>VHHPPSYVAHLASDFGVRVFQQVA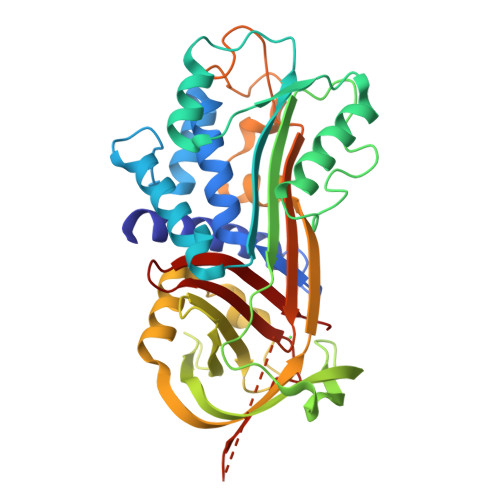QASKDRNVVFSPYGVASVLAMLQLTTGGETQQQIQAAMGFKIDDKGMAPALRHLYKELMGPWNKDEISTTDAIFVQRDLKLVQGFMPHFFRLFRSTVKQVDFSEVERARFIINDWVKTHTKGMISNLLGKGAVDQLTRLVLVNALYFNGQFKTPFPDSSTHRRLFHKSDGSTVSVPMMAQTNKFNYTEFTTPDGHYYDILELPYHGDTLSMFIAAPYEKEVPLSALTNILSAQLISHWKGNMTRLPRLLVLPKFSLETEVDLRKPLENLGMTDMFRQFQADFTSLSDQEPLHVAQALQKVKIEVNESGTVASSSTAVIVSARMAPEEIIMDRPFLFVVRHNPTGTVLFMGQVMEP[2x]>[2x]GSHMSLRHFLTLSDLTKQELENLIKRASELRKMQHAGEIYQPFVGRTLGMIFEKSSTRTRISFETGMGQFGGNAIFLSPNDTQLGRGEPLEDSARVISSMVDIIMIRTFGHEKVETFAEYSSVPIINALTDDYHPCQLLADMQTYYEHRGSIENKIVTWVGDGNNMCSSFMQAANQFGFELRVAAPYGF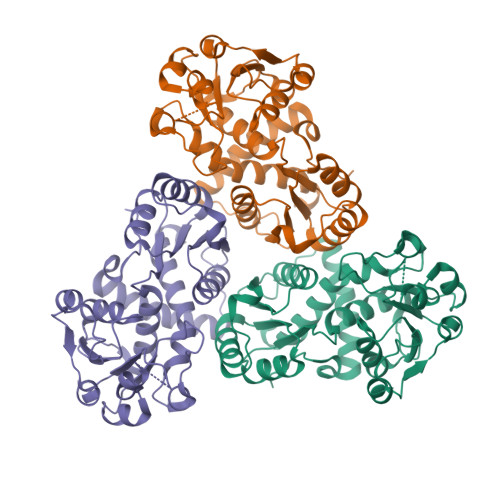EPDPKLMERFSHCVSLVENVQDAAKDANLIVTDVWASMGQESEQNTRARRFAPYQVTPSLLDKADPEVVFMHCLPAHRGEEISHDMLNDPRSVVWDEAENRLHAQKALMEFLLKDKIKI> TMAASQTSQTVASHVPFADLCSTLERIQKSKGRAEKIRHFREFLDSWRKFHDALHKNHKDVTDSFYPAMRLILPQLERERMAYGIKETMLAKLYIELLNLPRDGKDALKLLNYRTPTGTHGDAGDFAMIAYFVLKPRCLQKGSLTIQQVNDLLDSIASNNSAKRKDLIKKSLLQLITQSSALEQKWLIRMIIKDLKLGVSQQTIFSVFHNDAAELHNVTTDLEKVCRQLHDPSVGLSDISITLFSAFKPMLAAIADIEHIEKDMKHQSFYIETKLDGERMQMHKDGDVYKYFSRNGYNYTDQFGASPTEGSLTPFIHNAFKADIQICILDGEMMAYNPNTQTFMQKGTKFDIKRMVEDSDLQTCYCVFDVLMVNNKKLGHETLRKR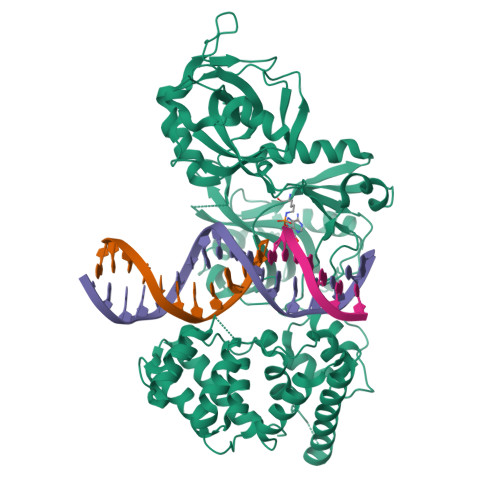YEILSSIFTPIPGRIEIVQKTQAHTKNEVIDALNEAIDKREEGIMVKQPLSIYKPDKRGEGWLKIKPEYVSGLMDELDILIVGGYWGKGSRGGMMSHFLCAVAEKPPPGEKPSVFHTLSRVGSGCTMKELYDLGLKLAKYWKPFHRKAPPSSILCGTEKPEVYIEPCNSVIVQIKAAEIVPSDMYKTGCTLRFPRIEKIRDDKEWHECMTLDDLEQLRGKASGKLASKHLYIGGD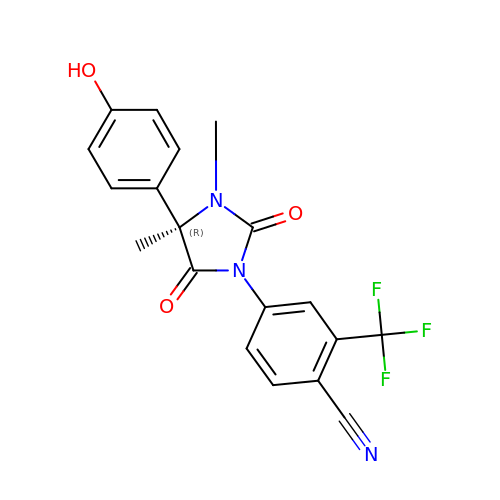4-[(4R)-4-(4-hydroxyphenyl)-3,4-dimethyl-2,5-dioxoimidazolidin-1-yl]-2-(trifluoromethyl)benzonitrile | C19 H14 F3 N3 O3 | IHPVXUVRRPAUIQ-GOSISDBHSA-N>[2x]PELSWSSANKYNIQVGDIMVRDVTSIASTSTYGDLLHVLRQTKLKFFPFVDTPDTNT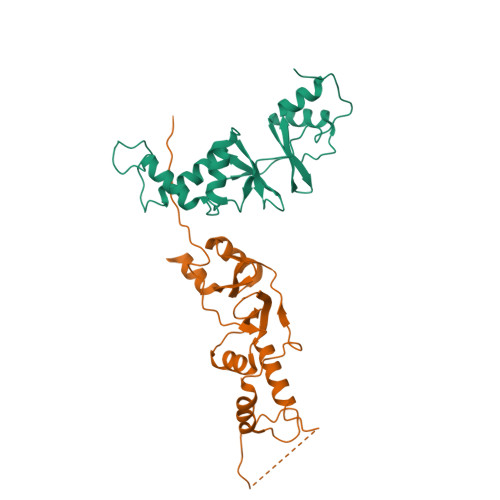LLGSIDRTEVEGLLQRRISAYRRQPAAAAEADEEGRNGETGASFTGEAESSFAYIDQEDAEGQQREGLEAVKVQTEDPRPPSPVPAEEPTQTSGIYQKKQKGTGQVASRFEEMLTLEEIYRWEQREKNVVVNFETCRIDQSPFQLVEGTSLQKTHTLFSLLGLDRAYVTSMGKLVGVVALAEIQAAIEGSYQK> MTTLRAFTCDDLFRFNNINLDPLTETYGIPFYLQYLAHWPEYFIVAEAPGGELMGYIMGKAEGSVAREEWHGHVTALSVAPEFRRLGLAAKLMELLEEISERKGGFFVDLFVRVSNQVAVNMYKQLGYSVY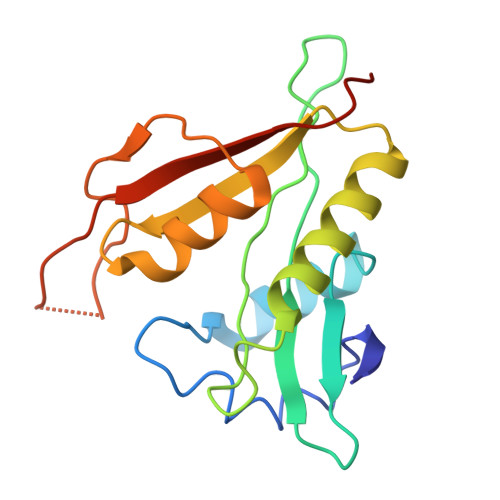RTVIEYYSASNGEPDEDAYDMRKALSRDTEKK>[4x]MEKSIKIGFIGLGAMGKPMAINLLKEGVTVYAFDLMEANVAAVVAQGAQACENNQKVAAASDIIFTSLPNAGIVETVMNGPGGVLSACKAGTVIVDMSSVSPSSTLKMAKVAAEKGIDYVDAPVSGGTKGAEA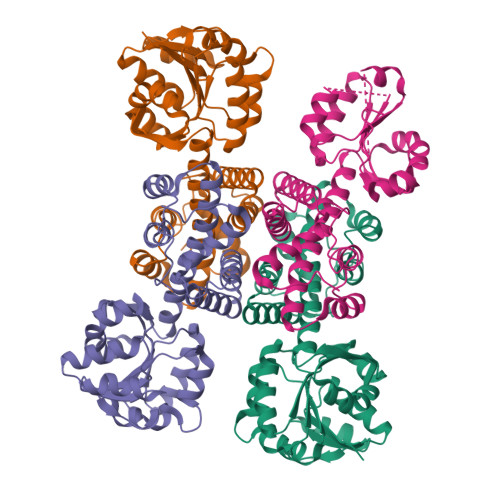GTLTIMVGASEAVFEKIQPVLSVIGKDIYHVGDTGAGDAVKIVNNLLLGCNMASLAEALVLGVKCGLKPETMQEIIGKSSGRSYAMEAKMEKFIMSGDFAGGFAMDLQHKDLGLALEAGKEGNVPLPMTAMATQIFEGGRAMGLGREDMSAVIKVWEQMTGVSVSGGQ The serine-rich repeat (SRR) glycoproteins of Gram-positive bacteria are an expanding family of microbial adhesins and virulence factors. Three of the SRR proteins (GspB of Streptococcus gordonii strain M99, Hsa of S. gordonii strain Challis, and SrpA of Streptococcus sanguinis strain SK36) bind human platelets through their interaction with glycocalicin, which is the carbohydrate-rich extracellular portion of the platelet membrane glycoprotein GPIbα. Among the best characterized of the SRR adhesins is GspB from S. gordonii, which has demonstrated binding affinity for the sialyl-T antigen carbohydrate decorating platelet glycoprotein GPIbα. Binding of these SRR adhesins to platelets is a high affinity process, with the interaction between GspB and glycocalicin having a KD of 2.38×10−8 M and appears to be a major factor in the pathogenesis of infective endocarditis, since the loss of GspB or Hsa expression results in a marked reduction in virulence.

We sought to identify the details of the interaction between GspBBR and the host receptor sialyl-T antigen. Dot blot assays using immobilized carbohydrates have demonstrated that GspB has high fidelity for sialyl-T antigen (i.e. NeuAcα(2–3)Galβ(1–3)GalNAc), one of the major carbohydrates on GPIbα, while Hsa binds to glycocalicin via either sialyl-T antigen or sialyllactose (Neu5Acα(2–6)Galβ(1–4)Glc). Site directed mutagenesis and in vivo studies in a rat model of infective endocarditis verified that this carbohydrate binding site within GspBBR mediates binding of S. gordonii strain M99 to sialyl-T antigen, the host carbohydrates of the platelet membrane receptor GPIbα, and intact platelets, and that this interaction is important for virulence. When PS2116 was tested with PS846 (M99ΔgspB) in this model, the strains had comparable but reduced densities within target tissues (as compared with WT M99), indicating that they were similarly reduced in virulence. These findings indicate that the predominant property of GspB contributing to the pathogenesis of endocarditis is its interaction with sialyl-T antigen.

>GPGSDTERPVVNVPSEITVYRGESFEYFATVTDNSNAFDLAKTVVRWLYSNQPGRGTEWLQYSVTQVGNQLKVRIFGNVPIDTTIGDYTRYVVATDAAGNVNATQTEMGNAAVDKTSVNGQFKLIIR[2x]The low-voltage activated T-type calcium channels regulate cellular excitability and oscillatory behavior of resting membrane potential which trigger many physiological events and have been implicated with many diseases. Here, we determine structures of the human T-type CaV3.3 channel, in the absence and presence of antihypertensive drug mibefradil, antispasmodic drug otilonium bromide and antipsychotic drug pimozide. The CaV3.3 channel consists of four repeated transmembrane domains, DI−DIV. Among them, the S1−S4 helices constitute the VSD; the S5 and S6 helices from all four domains form the ion-conducting pore; and the channel is formed in a domain-swapped fashion.

To improve the expression level and homogeneity of the protein sample, the N-terminal region (residues 1−42) and C-terminal region (residues 2065−2223) were truncated, and an incidental point mutation Glu523-to-Gln (E523Q) was included. Whole-cell patch-clamp experiment confirmed that these modifications on the CaV3.3 construct resulted in similar voltage dependency of the activation and steady-state inactivation compared to full-length wild-type CaV3.3. A total of 1135 residues were built into the final model. The selectivity filter ring contains four acidic residues, E357, E821, D1380, and D1678 (EEDD motif), one from each domain, and together they produce a strong negative charged area to attract cations and determines the selection specificity for Ca2+ ions. We identified a strong density inside the selectivity filter and close to the EEDD motif. We speculated that it represents a calcium ion, consistent with the previously observations in CaV channels structures. In addition, several phospholipids intrude into the central cavity from the fenestration sites around domain interfaces. The pore-lining helices (S6s) converged in the intracellular ends to form the intracellular gate. The pore profile calculated by the program HOLE34 indicated that this gate is closed in the apo state structure. CaV3.3 contains a long bended S6 helix from domain III, with a positive charged region protruding into the cytosol, which is critical for T-type CaV channel activation at low voltage.

> MAESASPPSSSAAAPAAEPGVTTEQPGPRSPPSSPPGLEEPLDGADPHVPHPDLAPIAFFCLRQTTSPRNWCIKMVCNPWFECVSMLVILLNCVTLGMYQPCDDMDCLSDRCKILQVFDDFIFIFFAMEMVLKMVALGIFGKKCYLGDTWNRLDFFIVMAGMVEYSLDLQNINLSAIRTVRVLRPLKAINRVPSMRILVNLLLDTLPMLGNVLLLCFFVFFIFGIIGVQLWAGLLRNRCFLEENFTIQGDVALPPYYQPEEDDEMPFICSLSGDNGIMGCHEIPPLKEQGRECCLSKDDVYDFGAGRQDLNASGLCVNWNRYYNVCRTGSANPHKGAINFDNIGYAWIVIFQVITLEGWVEIMYYVMDAHSFYNFIYFILLIIVGSFFMINLCLVVIATQFSETKQREHRLMLEQRQRYLSSSTVASYAEPGDCYEEIFQYVCHILRKAKRRALGLYQALQSRRQALGPEAPAPAKPGPHAKEPRHYHGKTKGQGDEGRHLGSRHCQTLHGPASPGNDHSGRELCPQHSPLDATPHTLVQPIPATLASDPASCPCCQHEDGRRPSGLGSTDSGQEGSGSGSSAGGEDEADGDGARSSEDGASSELGKEEEEEEQADGAVWLCGDVWRETRAKLRGIVDSKYFNRGIMMAILVNTVSMGIEHHEQPEELTNILEICNVVFTSMFALEMILKLAAFGLFDYLRNPYNIFDSIIVIISIWEIVGQADGGLSVLRTFRLLRVLKLVRFMPALRRQLVVLMKTMDNVATFCMLLMLFIFIFSILGMHIFGCKFSLRTDTGDTVPDRKNFDSLLWAIVTVFQILTQEDWNVVLYNGMASTSPWASLYFVALMTFGNYVLFNLLVAILVEGFQAEGDANRSYSDEDQSSSNIEEFDKLQEGLDSSGDPKLCPIPMTPNGHLDPSLPLGGHLGPAGAAGPAPRLSLQPDPMLVALGSRKSSVMSLGRMSYDQRSLSSSRSSYYGPWGRSAAWASRRSSWNSLKHKPPSAEHESLLSAERGGGARVCEVAADEGPPRAAPLHTPHAHHIHHGPHLAHRHRHHRRTLSLDNRDSVDLAELVPAVGAHPRAAWRAAGPAPGHEDCNGRMPSIAKDVFTKMGDRGDRGEDEEEIDYTLCFRVRKMIDVYKPDWCEVREDWSVYLFSPENRFRVLCQTIIAHKLFDYVVLAFIFLNCITIALERPQIEAGSTERIFLTVSNYIFTAIFVGEMTLKVVSLGLYFGEQAYLRSSWNVLDGFLVFVSIIDIVVSLASAGGAKILGVLRVLRLLRTLRPLRVISRAPGLKLVVETLISSLKPIGNIVLICCAFFIIFGILGVQLFKGKFYHCLGVDTRNITNRSDCMAANYRWVHHKYNFDNLGQALMSLFVLASKDGWVNIMYNGLDAVAVDQQPVTNHNPWMLLYFISFLLIVSFFVLNMFVGVVVENFHKCRQHQEAEEARRREEKRLRRLEKKRRKAQRLPYYATYCHTRLLIHSMCTSHYLDIFITFIICLNVVTMSLEHYNQPTSLETALKYCNYMFTTVFVLEAVLKLVAFGLRRFFKDRWNQLDLAIVLLSVMGITLEEIEINAALPINPTIIRIMRVLRIARVLKLLKMATGMRALLDTVVQALPQVGNLGLLFMLLFFIYAALGVELFGKLVCNDENPCEGMSRHATFENFGMAFLTLFQVSTGDNWNGIMKDTLRDCTHDERSCLSSLQFVSPLYFVSFVLTAQFVLINVVVAVLMKHLDDSNKEAQEDAEMDAELELEMAHGLGPGPRLPTGSPGAPGRGPGGAGGGGDTEGGLCRRCYSPAQENLWLDSVSLIIKDSLEGELTIIDNLSGSIFHHYSSPAGCKKCHHDKQEVQLAETEAFSLNSDRSSSILLGDDLSLEDPTACPPGRKDSKGELDPPEPMRVGDLGECFFPLSSTAVSPDPENFLCEMEEIPFNPVRSWLKHDSSQAPPSPFSPDASSPLLPMPAEFFHPAVSASQKGPEKGTGTGTLPKIALQGSWASLRSPRVNCTLLRQATGSDTSLDASPSSSAGSLQTTLEDSLTLSDSPRRALGPPAPAPGPRAGLSPAARRRLSLRGRGLFSLRGLRAHQRSHSSGGSTSPGCTHHDSMDPSDEEGRGGAGGGGAGSEHSETLSSLSLTSLFCPPPPPPAPGLTPARKFSSTSSLAAPGRPHAAALAHGLARSPSWAADRSKDPPGRAPLPMGLGPLAPPPQPLPGELEPGDAASKRKR> GTSTQTKAGSLTIVGTGIESIGQMTLQALSYIEAAAKVFYCVIDPATEAFILTKNKNCVDLYQYFDNGKSRLNTYTQMSELMVREVRKGLDVVGVFYGHPGVFVNPSHRALAIAKSEGYRARMLPGVSAEDCLFADLCIDPSNPGCLTYEASDFLIRDRPVSIHSHLVLFQVGCVGIADFNFTGFDNNKFGVLVDRLEQEYGAEHPVVHYIAAMMPHQDPVTDKYTVAQLREPEIAKRVGGVSTFYIPPKARKASNLDIIRRLELLPAGQVPDKKARIYPANQWEPDVPEVEPYRPSDQAAIAQLADHAPPEQYQPLATSKAMSDVMTKLALDPKALADYKADHRAFAQSVPDLTPQERAALELGDSWAIRCAMKNMPSSLLDAARESGEEASQNGFPWVIVVGVIGVIG

While chemical methylation of an amide bond uses a strong base to generate the imidate, OphA, the precursor protein of the fungal peptide macrocycle omphalotin A, self-hypermethylates amides at pH 7 using S-adenosyl methionine (SAM) as cofactor. Omphalotin A derives from the C terminus of the OphA protein, and it is the OphA protein that methylates its own C terminus using S-adenosyl methionine (SAM). The structure of OphA reveals a complex catenane-like arrangement in which the peptide substrate is clamped with its amide nitrogen aligned for nucleophilic attack on the methyl group of SAM. Here, we report the structure of the peptide amide methyltransferase OphA including complexes with cofactor [SAM and S-adenosyl homocysteine (SAH)], cofactor analog, substrate, and product.

Mutants Y63F, Y66F, Y76F, R72A, R72K, Y98A, Y98F, Q172A, and W400A of OphAΔC6 were expressed in E. coli. Y63F, Y66F, Y76F, R72A, Y98A, and W400A were incubated with SAM and analyzed. The peptide carbonyl at i−3 hydrogen-bonds to the side chain of Tyr63, at i−2 to the side chain of Tyr98, and at i−1 to both Tyr66 and Tyr76. Y66F retains activity, and Tyr76, although within 4 Å of the carbonyl, has a Bürgi-Dunitz (44°) angle incompatible with attack, so both possibilities were discarded. Both Tyr66 and Tyr76 are, however, well positioned to stabilize the resulting tetrahedral carbon by hydrogen bonding. The resulting negatively charged oxygen of the imidate would be stabilized by hydrogen bonds to Tyr66 and Tyr76.One well-studied efflux pump is the tripartite assembly formed in E. coli by the outer membrane protein TolC, the periplasmic protein AcrA, and the inner membrane protein AcrB, which uses proton motive force to translocate acridine and other drug-like compounds. TolC is a homotrimeric channel assembly with a transmembrane spanning portion and an extensive periplasmic domain that has two distinct sections: an outer membrane proximal subdomain in which 12 helices pack to form a hollow cylinder, and a distal subdomain where 12 helices form conventional coiled coils that curve to meet at a juncture that occludes the channel for all but the smallest ions. The interaction of adjacent coiled-coil pairs is stabilized in part through hydrogen bonds and salt bridges, and mutation of the residues participating in these interactions causes the channel to become permissive to the diffusion of ions across the membrane in vitro (Andersen et al., 2002) and to the entry of antibiotic in vivo (Augustus et al., 2004). In this study, we have examined a network of hydrogen-bonding interactions at the aperture end of the TolC which, when mutated, partially opens the channel so that it becomes leaky to bulky molecules in vivo.

We have solved the crystal structure of the Y362F, R367E mutant in two crystalline forms at 3.2 and 3.3 Å resolution. Corroborating the in vivo effects, the crystal structures of the double mutant reveal significant repacking of the helices in the distal helical domain that partially opens the channel, relative to the closed structure. The crystal structures of the double mutant show that three of the six pairs of coiled coils move radially outward from the central molecular axis of the trimer in comparison with the closed-state form, widening up the periplasmic lumen of the channel like the iris mechanism of a camera. In one of the crystal forms (spacegroup C2), neighboring TolC trimers pack tightly so that the exposed loop regions of the coiled coils H3/H4 and H7/H8 pair in a self-complementary fashion, and the H3/H4 loops form a hydrogen-bonding network. This crystal form has a greater displacement of the helical pairs H7/H8 compared to the P212121 form. In the C2 form, the maximal displacement of the H7 helix on the leading edge is over 11 Å in the case of the chain B, and the corresponding maximal displacement of the lagging H8 helix from its original position in the resting state is roughly 4.5 Å. We note that a similar interpenetration takes place in the C2 crystal form of the TolC mutant, where H3/H4 helices pack against each other in symmetry-related molecules. It is thus plausible that the shallow intermeshing of TolC trimers may mimic its interactions with AcrB in the acridine efflux drug assembly, where backbone-mediated interactions play a role in the engagement of AcrB and TolC static helices H3/H4. The asymmetry of the open-state structures is also reflected in the exposed surface of the three grooves that putatively engage AcrA.

>[3x]MRKLLPILIGLSLSGFSSLSQAENLMQVYQQARLSNPELRKSAADRDAAFEKINEARSPLLPQLGLGADYTYSNGYRDANGINSNATSASLQLTQSIFDMSKWRALTLQEKAAGIQDVTYQTDQQTLILNTATAYFNVLNAIDVLSYTQAQKEAIYRQLDQTTQRFNVGLVAITDVQNARAQYDTVLANELTARNNLDNAVEQLRQITGNYYPELAALNVENFKTDKPQPVNALLKEAEKRNLSLLQARLSQDLAREQIRQAQDGHLPTLDLTASTGISDTSYSGSKTRGAAGTQYDDSNMGQNKVGLSFSLPIYQGGMVNSQVKQAQYNFVGASEQLESAHRSVVQTVRSSFNNINASISSINAYKQAVVSAQSSLDAMEAGFSVGTETIVDVLDATTTLYNAKQELANARYNYLINQLNIKSALGTLNEQDLLALNNALSKPVSTNPELEHHHHHHHH Clostridium thermocellum has extensive potential in lignocellulose biorefineries as an environmentally prominent, thermophilic, cellulolytic bacterium. Previously, five putative sugar transporters, denoted A to D and L and belonging to the ABC transport systems group, were identified in the genome of C. thermocellum, and the solute-binding lipoproteins (SBP) of these ABC transporters were shown to bind different dextrins by isothermal titration calorimetry (ITC) assays. To gain insight into the structural mechanism of the transporter specificities, 11 crystal structures, both alone and in complex with appropriate saccharides, were solved for all 5 putative sugar-binding proteins, thus providing detailed specific interactions between the proteins and the corresponding saccharides. Combined genetic, biophysical, and structural studies have provided solid evidence that transporter A and transporter B are the major glucose and cellodextrin transporters, respectively, among the five potential sugar transporters in C. thermocellum.

Four SBPs, denoted cellodextrin-binding proteins A to D (CbpA to CbpD), were shown to bind to glucose and/or different lengths of cellodextrins; and one SBP, denoted laminaribiose-binding protein (Lbp), was shown to bind laminaribiose. The structure of Lbp was determined to 1.50 Å resolution. Although no sugar was added during crystallization, a clear electron density of a small molecular substrate was observed in the structure. However, neither laminaribiose nor cellobiose can fit into the density. Considering that Lbp has about 35% sequence identity with nucleoside-binding proteins as shown by a BLAST search, we tried to fit different nucleotides and found that guanosine fits well into the density. Furthermore, the ΔtransporterL strain grew well in the medium with laminaribiose as the sole carbon source. Further studies, however, are still required to elucidate the interaction of Lbp with laminaribiose and whether it can function in laminaribiose transport.

>[2x]SKNSGNNSNNSSNNNSSNNTGGKKIKIGMVTDVGGVNDGSFNQSAWEGLQRAQKELGVEVRYAESATDADYAPNIEAFIDEGYDLIICVGYMLADATRKAAEANPNQKFAIIDDASIDLPNVTCLMFEQSQASYLVGLVAGKMTKTNKVGFVVGMVSQTMNEFGYGYLAGVKDANPNATILQFNANSFSSTETGKSAATTMITNGADVIFHAAGGTGLGVIEGCKDAGKWAIGVDSDQSPLAPENILTSAMKRVDNACFDIAKAVKEGNVKPGIITYDLKSAGVDIAPTTTNLPKEVLDYVNQAKQDIINGKITVPKTKAEFEAKYGNIYELDD>MATATEQWVLVEMVQALYEAPAYHLILEGILILWIIRLLFSKTYKLQERSDLTVKEKEELIEEWQPEPLVPPVPKDHPALNYNIVSGPPSHKTVVNGKECINFASFNFLGLLDNPRVKAAALASLKKYGVGTCGPRGFYGTFDVHLDLEDRLAKFMKTEEAIIYSYGFATIASAIPAYSKRGDIVFVDRAACFAIQKGLQASRSDIKLFKHNDMADLERLLKEQEIEDQKNPRKARVTRRFIVVEGLYMNTGTICPLPELVKLKYKYKARIFLEESLSFGVLGEHGRGVTEHYGINIDDIDLISANMENALASIGGFCCGRSFVIDHQRLSGQGYCFSASLPPLLAAAAIEALNIMEENPGIFAVLKEKCGQIHKALQGISGLKVVGESLSPAFHLQLEESTGSREQDVRLLQEIVDQCMNRSIALTQARYLEKEEKCLPPPSIRVVVTVEQTEEELERAASTIKEVAQAVLL[2x];>[2x]MRPEPGGCCCRRTVRANGCVANGEVRNGYVRSSAAAAAAAAAGQIHHVTQNGGLYKRPFNEAFEETPMLVAVLTYVGYGVLTLFGYLRDFLRYWRIEKCHHATEREEQKDFVSLYQDFENFYTRNLYMRIRDNWNRPICSVPGARVDIMERQSHDYNWSFKYTGNIIKGVINMGSYNYLGFARNTGSCQEAAAKVLEEYGAGVCSTRQEIGNLDKHEELEELVARFLGVEAAMAYGMGFATNSMNIPALVGKGCLILSDELNHASLVLGARLSGATIRIFKHNNMQSLEKLLKDAIVYGQPRTRRPWKKILILVEGIYSMEGSIVRLPEVIALKKKYKAYLYLDEAHSIGALGPTGRGVVEYFGLDPEDVDVMMGTFTKSFGASGGYIGGKKELIDYLRTHSHSAVYATSLSPPVVEQIITSMKCIMGQDGTSLGKECVQQLAENTRYFRRRLKEMG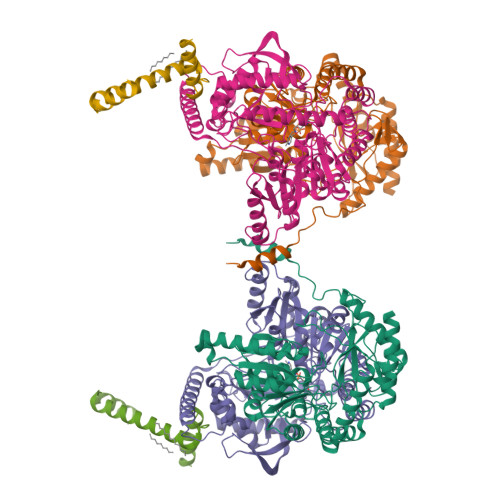FIIYGNEDSPVVPLMLYMPAKIGAFGREMLKRNIGVVVVGFPATPIIESRARFCLSAAHTKEILDTALKEIDEVGDLLQLKYSRHRL;>MAGMALARAWKQMSWFYYQYLLVTALYMLEPWERTVFNSMLVSIVGMALYTGYVFMPQHIMAILHYFEIVQ[2x]>[2x]GDNDAIYYPVGDVDIERGGPALEVGEEDVLVA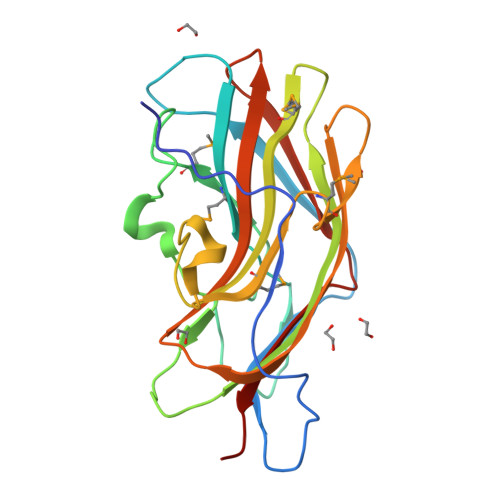RSFNEEDYVLDTIAQYPNDPTLGKLTFMIDLKNQQKDQNVADFNGVGKSKLTMSLGYKDGNYPSESQVPIYTSQDVTAKYAVKLRLKGELLVSGDEWMIDYVYAQLASLFQPYPPANFPEVFMCKGGMKLGTFDSFRRTCTFDITYDRSDLSFSQLYFNLFINLAGQKRENRVRLRIDKESYFELYEQSEEM> ANTSSAYNSVYDFLRYHDRGDGLTVNGKTSYSIDQAAAQITRENVSWNGTNVFGKSANLTFKFLQSVSSIPSGDTGFVKFNAEQIEQAKLSLQSWSDVANLTFTEVTGNKSANITFGNYTRDASGNLDYGTQAYAYYPGNYQGAGSSWYNYNQSNIRNPGSEEYGRQTFTHEIGHALGLAHPGEYNAGEGDPSYNDAVYAEDSYQFSIASYWGENETGADYNGHYGGAPMIDDIAAIQRLYGANMTTRTGDSVYGFNSNTDRDFYTATDSSKALIFSVWDAGGTDTFDFSGYSNNQRINLNEGSFSDVGGLKGNVSIAHGVTIENAIGGSGNDILVGNSADNILQGGAGNDVLYGGAGADTLYGGAGRDTFVYGSGQDSTVAAYDWIADFQKGIDKIDLSAFRNEGQLSFVQDQFTGKGQEVMLQWDAANSIT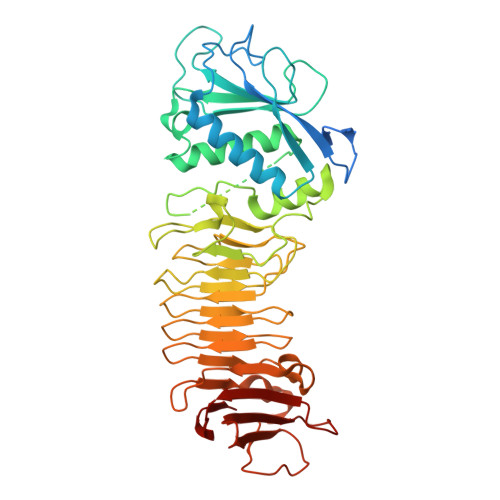NLWLHEAGHSSVDFLVRIVGQAAQSDIIV>MAAACRSVKGLVAVITGGASGLGLATAERLVGQGASAVLLDLPNSGGEAQAKKLGNNCVFAPADVTSEKDVQTALALAKGKFGRVDVAVNCAGIAVASKTYNLKKGQTHTLEDFQRVLDVNLMGTFNVIRLVAGEMGQNEPDQGGQRGVIINTASVAAFEGQVGQAAYSASKGGIVGMTLPIARDLAPIGIRVMTIAPGLFGTPLLTSLPEKVRNFLASQVPFPSR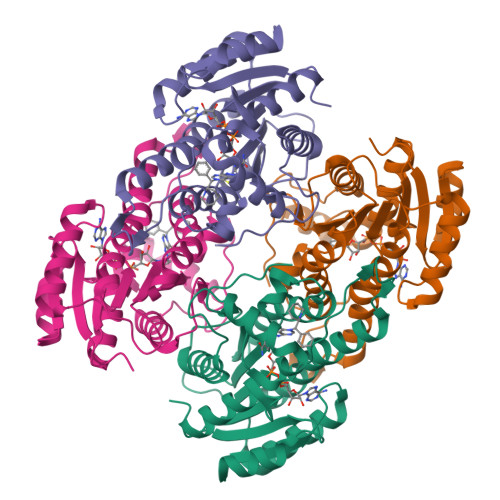LGDPAEYAHLVQAIIENPFLNGEVIRLDGAIRMQP[4x]>[2x]MPVTINNFNYNDPIDNNNIIMMEPPFARGTGRYYKAFKITDRIWIIPERYTFGYKPEDFNKSSGIFNRDVCEYYDPDYLNTNDKKNIFLQTMIKLFNRIKSKPLGEKLLEMIINGIPYLGDRRVPLEEFNTNIASVTVNKLISNPGEVERKKGIFANLIIFGPGPVLNENETIDIGIQNHFASREGFGGIMQMKFCPEYVSVFNNVQENKGASIFNRRGYFSDPALILMHQLIYVLHGLYGIKVDDLPIVPNEKKFFMQSTDAIQAEELYTFGGQDPSIITPSTDKSIYDKVLQNFRGIVDRLNKVLVCISDPNININIYKNKFKDKYKFVEDSEGKYSIDVESFDKLYKSLMFGFTETNIAENYKIKTRASYFSDSLPPVKIKNLLDNEIYTIEEGFNISDKDMEKEYRGQNKAINKQAYEEISKEHLAVYKIQMCKSVKAPGICIDVDNEDLFFIADKNSFSDDLSKNERIEYNTQSNYIENDFPINELILDTDLISKIELPSENTESLTDFNVDVPVYEKQPAIKKIFTDENTIFQYLYSQTFPLDIRDISLTSSFDDALLFSNKVYSFFSMDYIKTANKVVEAGLFAGWVKQIVNDFVIEANKSNTMDKIADISLIVPYIGLALNVGNETAKGNFENAFEIAGASILLEFIPELLIPVVGAFLLESYIDNKNKIIKTIDNALTKRNEKWSDMYGLIVAQWLSTVNTQFYTIKEGMYKALNYQAQALEEIIKYRYNIYSEKEKSNINIDFNDINSKLNEGINQAIDNINNFINGCSVSYLMKKMIPLAVEKLLDFD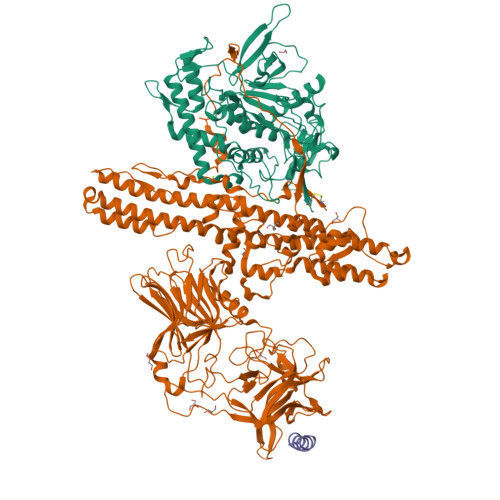NTLKKNLLNYIDENKLYLIGSAEYEKSKVNKYLKTIMPFDLSIYTNDTILIEMFNKYNSEILNNIILNLRYKDNNLIDLSGYGAKVEVYDGVELNDKNQFKLTSSANSKIRVTQNQNIIFNSVFLDFSVSFWIRIPKYKNDGIQNYIHNEYTIINCMKNNSGWKISIRGNRIIWTLIDINGKTKSVFFEYNIREDISEYINRWFFVTITNNLNNAKIYINGKLESNTDIKDIREVIANGEIIFKLDGDIDRTQFIWMKYFSIFNTELSQSNIEERYKIQSYSEYLKDFWGNPLMYNKEYYMFNAGNKNSYIKLKKDSPVGEILTRSKYNQNSKYINYRDLYIGEKFIIRRKSNSQSINDDIVRKEDYIYLDFFNLNQEWRVYTYKYFKKEEMKLFLAPIYDSDEFYNTIQIKEYDEQPTYSCQLLFKKDEESTDEIGLIGIHRFYESGIVFEEYKDYFCISKWYLKEVKRKPYNLKLGCNWQFIPKDEGWTE;> GESQEDMFAKLKEKLFNEINK>[2x]RTGSYGDVNRVDTTGASSKSAKPEKLNYSGVAASRKIAERDLQSMDRYKALIKKVGQKLSVDPAVIAGIISRESHAGKALRNGWGDNGNGFGLMQVDRRSHKPVGEWNGERHLMQGTEIL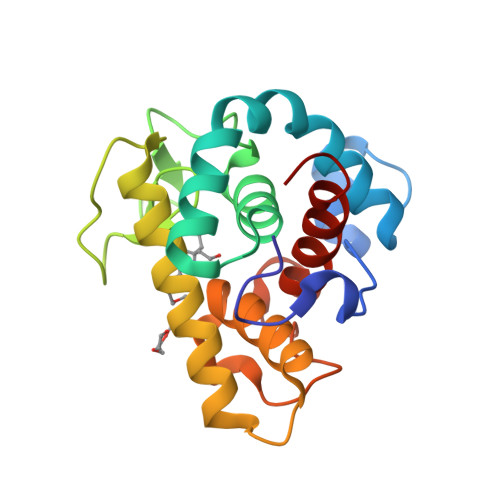ISMIKAIQKKFPRWTKEQQLKGGISAYNAGPGNVRSYERMDIGTTHDDYANDVVARAQYYKQHGY> GCAGGGCAAGGCCCAGUCCCG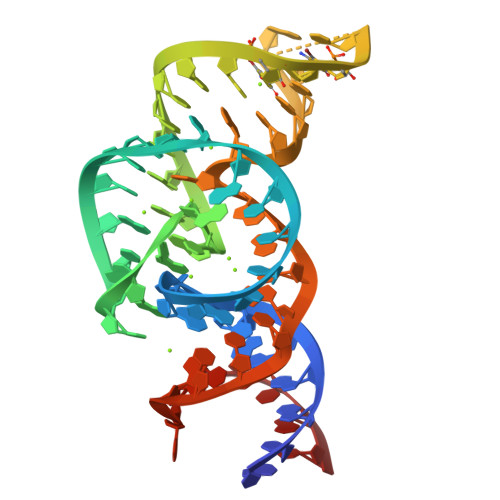UGCAAGCCGGGACCGCCCCGGGGCGCGGCGCUCAUUCCUGC>DLSQCDREPIHLLGGIQSHGVLLAFRGPDRLLEVVSANAQALLGRPPETLLGQPVGRVLPAEVLAQWEPLVARGSVRVVLPAGAYRALLHESDGLTVLELEPAELQPGMEETALEVVRRLVSPLAGVKGTQALLQTAADTVRALTGFDRVMVYRFDADWHGEVLAESKRGGMDGFLGMHFPATDIPVQARALYTRNPLRLIADARARPVPLLPPVVPALGRPLDLSNSALRSVSPVHLEYLRNMGVGASFSLSLLKEGVLWGLIACHHLEPL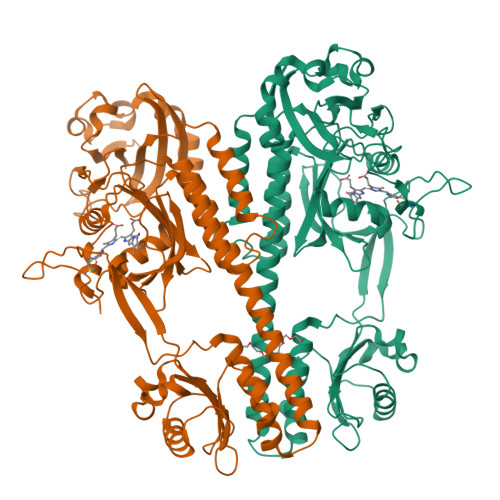HISHERRRACEVLTQLLALQLSAEERAAEASEDAHRAALLGQLATAMGEGGTLEEVLEKESERVLALTGAAGVALLLGEEPLLVGCTPAQDEVEALVAWLATQPFQTSFHTDRLGTVYPPLAARADVAAGILAVRLAPAAARFAIWFRPEVARTISWAGNPRKPAEPEPGHQRLHPRGSFQAWEETVRDTSLPWKRADLGAAEGFRGALV[2x]> MGQAWQEASDNCFMDSDIKVLEDQFDEIIVDIATKRK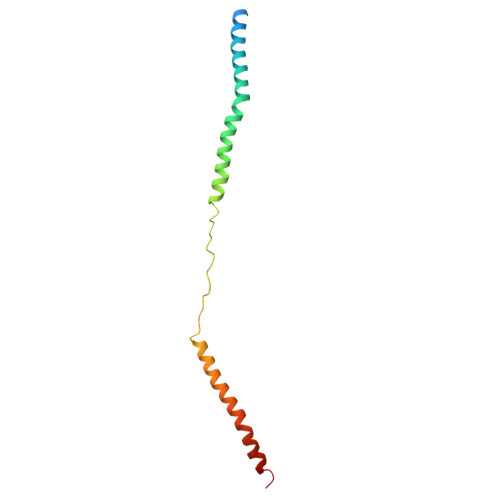QYPRKILECVIKTIKAKQEILKQYHPVVHPLDLKYDPDPAPHMENLKCRGETVAKEISEAMKSLPALIEQGEGFSQVLR> MDPDELPLDEHCERLPYDASKWEFPRDRLKLGKPLGRGAFGQVIEADAFGIDKTATCRTVAVKMLKEGATHSEHRALMSELKILIHIGHHLNVVNLLGACTKPGGPLMVIVEFCKFGNLS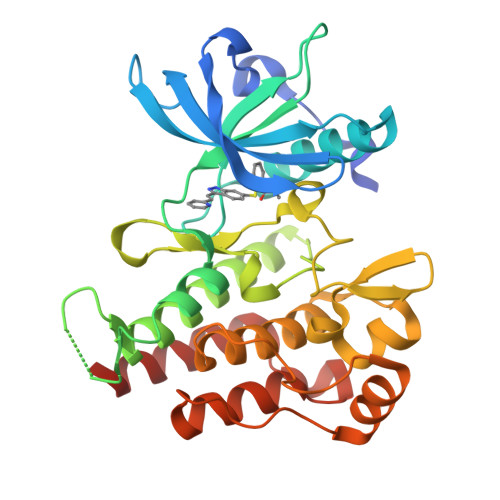TYLRSKRNEFVPYKVAPEDLYKDFLTLEHLICYSFQVAKGMEFLASRKCIHRDLAARNILLSEKNVVKICDFGLARDIYKDPDYVRKGDARLPLKWMAPETIFDRVYTIQSDVWSFGVLLWEIFSLGASPYPGVKIDEEFCRRLKEGTRMRAPDYTTPEMYQTMLDCWHGEPSQRPTFSELVEHLGNLLQANAQQD>XADEIAKAQVARPGGDTIFGKIIRKEIPAKIIFEDDRCLAFHDISPQAPTHFLVIPKKHISQISVAEDDDESLLGHLMIVGKKCAADLGLN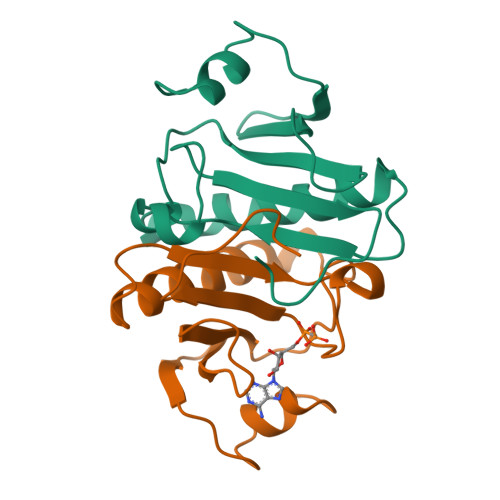KGYRMVVNEGSDGGQSVYHVHLHVLGGRQMHWPPG[2x]>GAMAGKKVLIVYAHQEPKSFNGSLKNVAVDELSRQGCTVTVSDLYAMNFEPRATDKDITGTLSNPEVFNYGVETHEAYKQRSLASDITDEQKKVREADLVIFQFPLYWFSVPAILKGWMDRVLCQGFAFDIPGFYDSGLLQGKLALLSVTTGGTAEMYTKTGVNGDSRYF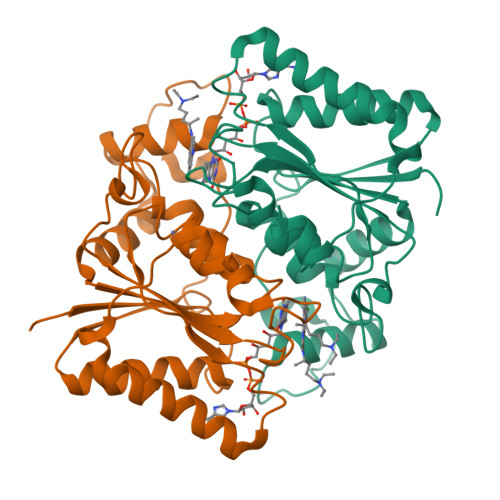LWPLQHGTLHFCGFKVLAPQISFAPEIASEEERKGMVAAWSQRLQTIWKEEPIPCTAHWHFGQ[2x]> MAHLKKRNRLK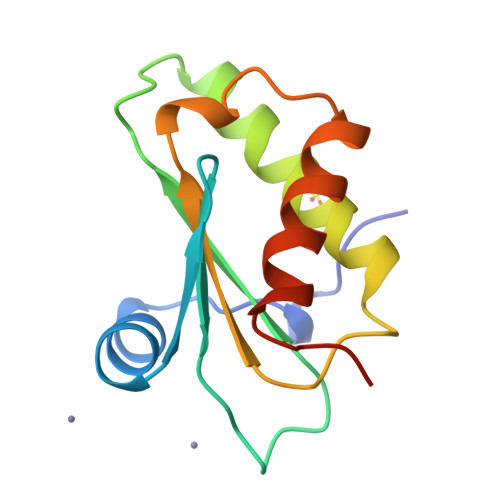KNEDFQKVFKHGTSVANRQFVLYTLDQPENDELRVGLSVSKKIGNAVMRNRIKRLIRQAFLEEKERLKEKDYIIIARKPASQLTYEETKKSLQHLFRKSSLYKKSSSK> GNTLVVLHKSGLLEITLKTKELIRQNQATQAELDQLKEQTQMFIEATKSRA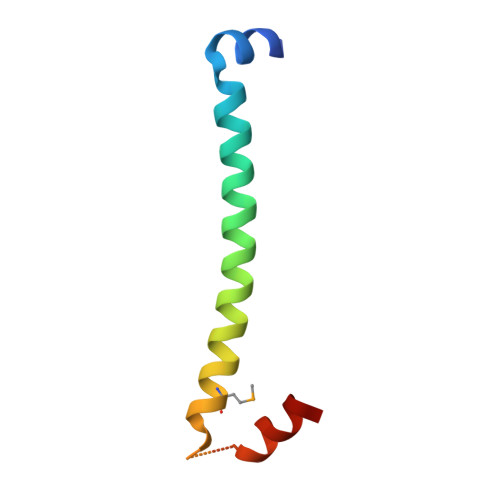PQAWAKLQASLTS> ASGLFITNEGNFQYSNATLSYYDPATCEVENEVFYRANGFKLGDVAQSMVIRDGIGWIVVNNSHVIFAIDINTFKEVGRITGFTSPRYIHFLSDEKAYVTQIWDYRIFIINPKTYEITGYIECPDMDMESGSTEQMVQYGKYVYVNCWSYQNRILKIDTETDKVVDELTIGIQPTSLVMDKYNKMWTITDGGYEGSPYGYEAPSLY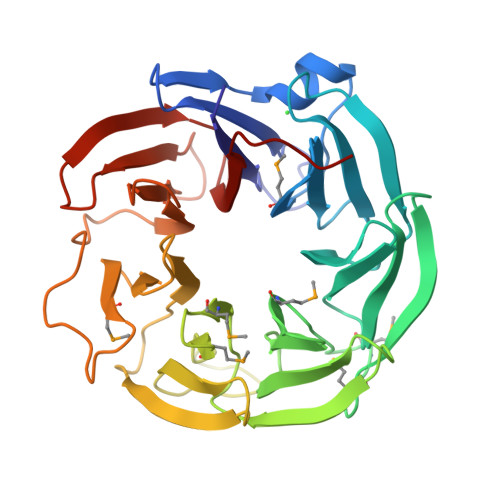RIDAETFTVEKQFKFKLGDWPSEVQLNGTRDTLYWINNDIWRMPVEADRVPVRPFLEFRDTKYYGLTVNPNNGEVYVADAIDYQQQGIVYRYSPQGKLIDEFYVGIIPGAFCWKLEHHHHHH>MVNVTVAYQTSAEPAKVAQADNTFAKESGATVDWRKFDSGASIVRALASGDVQIGNLGSSPLAVAASQQVPIEVFLLASKLGNSEALVVKKTISKPEDLIGKRIAVPFISTTHYSLLAALKHWGIKPGQVEIVNLQPPAIIAAWQRGDIDGAYVWAPAVNALEKDGKVLTDSEQVGQWGAPTLDVWVVRKDFAEKHPEVVKAFAKSAIDAQQPYIANPDVWLKQPENISKLARLSGVPEGDVPGLVKGNTYLTPQQQTAELTGPVNKAIIDTA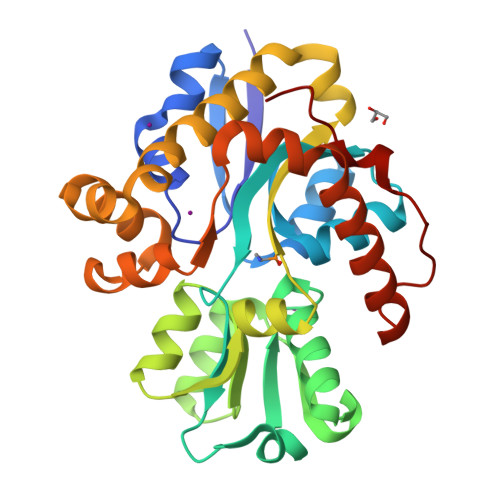QFLKEQGKVPAVANDYSQYVTSRFV[2x]The alg operon also encodes a periplasmic lyase, AlgL. Characterization of this enzyme in vitro demonstrated that it preferentially degrades nonacetylated polymannuronate (polyM) via a ß-elimination mechanism. The structure reveals that AlgL adopts an (α/α)5 toroid fold with five pairs of antiparallel α-helices. Our in vivo studies demonstrate that AlgL does not associate with other alginate biosynthetic proteins and functions as a periplasmic homeostasis enzyme to clear the periplasm of accumulated alginate to prevent cell lysis.

To investigate how the H202A and K66A active site mutants might affect enzymatic activity and account for the discrepancies between in vivo phenotypes and in vitro catalytic activities observed, we determined the structures of the AlgL H202A and K66A variants. K66A and Y259F retained approximately 1% and 30% catalytic efficiency, respectively, compared with WT. Although K66A retains enzymatic activity and the strain does not demonstrate an in vivo growth defect, some cells were observed to display aberrant cell membrane phenotypes by TEM. Comparison of the K66A variant with WT AlgL revealed that the two structures are highly similar with a Cα RMSD of 0.352 Å. However, residues 66 to 81 within the lid-loop region of K66A AlgL could not be built into the model, suggesting that the lid-loop region in this mutant is flexible. Similarly, we were unable to observe any corresponding density for the mannuronate substrate soaked into the crystal prior to data collection. K66 interacts with the sugar ligand and appears to contribute to loop enclosure in the WT enzyme. Mutation of K66 and the resulting flexibility of the lid-loop region suggest that K66 in AlgL is important for priming the enzyme for catalysis by locking the lid-loop in a closed conformation after substrate binding. This could explain the abnormal cellular morphology observed in vivo in the K66A strain and the reduced enzymatic efficiency of this mutant variant in vitro.

> MHHHHHHSSGRENLYFQGADLVPPPGYYAAVGERKGSAGSCPAVPPPYTGSLVFTSAYEGSDSARATLNVKAEKTFRSQIKDITDMERGATKLVTQYMRSGRDGDLACALNWMSAWARAGALQSDDFNHTGKSMRKWALGSLSGAYMRLKFSSSRPLAAHAEQSREIEDWFARLGTQVVRDWSGLPLKKINNHSYWAAWSVMSTAVVTNRRDLFDWAVSEFKVAANQVDEQGFLPNELKRRQRALAYHNYALPPLAMIAAFAQVNGVDLRQENHGALQRLAERVMKGVDDEETFEEKTGEDQDMTDLKVDNKYAWLEPYCALYRCEPKMLEAKKDREPFNSFRLGGEVTRVFS> STMPLAELGA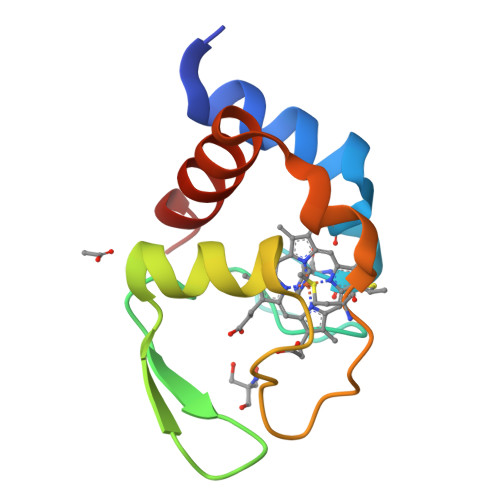RLYREKACFSCHSIDGSRLVGPSFKGLYGSTRTFEDGTTAVADENYLRESILQPGAKVVQGYPNVMPASYASLSEREVAALIEFIKQQQ>VMYYGKGDVFAYRTYLKPLTGVRTIPESPFSGRDHILFGVNVK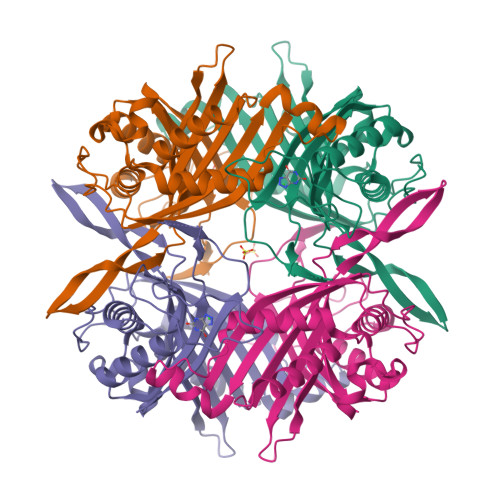ISVGGTKLLTSFTKGDNSLVVATDSMKNFIQKHLASYTGTTIEGFLEYVATSFLKKYSHIEKISLIGEEIPFETTFAVKNGNRAASELVFKKSRNEYATAYLNMVRNEDNTLNITEQQSGLAGLQLIKVSGNSFVGFIRDEYTTLPEDSNRPLFVYLNIKWKYKNTEDSFGTNPENYVAAEQIRDIATSVFHETETLSIQHLIYLIGRRILERFPQLQEVYFESQNHTWDKIVEEIGESEGKVYTEPRPPYGFQCFTVTQEDLPHENILMFSDE[4x]>[2x]MLYIDEFKEAIDKGYILGDTVAIVRKNGKIFDYVLPHEKVRDDEVVTVERVEEVMVELDKLEHHHHHH;> GSHMLKDFGKKIKSLRLEKGLTKEAVCLDESQLSTRQLTRIESGQSTPTLNKAVYIAGRLGVTLGYLTD

Within S. pyogenes, Prx functions to inhibit the quorum-sensing receptor-signal pair ComRS, the master regulator of natural competence, or the ability to uptake endogenous DNA. ComR is a quorum-sensing receptor and a transcription factor that belongs to the Rgg subgroup of the RRNPP protein family, many of which regulate virulence in pathogenic Streptococcus species. ComR is a monomer that contains a DNA-binding domain (DBD) packed against a tetratricopeptide repeat (TPR) domain. Specifically, Prx binds directly to the apo-form of ComR preventing DNA binding in vitro and acts as a repressor of the S. pyogenes competence regulon in vivo.

Despite not being able to obtain an X-ray crystal structure of Prx in complex with full-length ComR, we were able to cocrystallize Prx with the DBD of ComR. DBD:Prx cocrystals were obtained with both purified minimal DBD bound to Prx and after in situ proteolysis with full-length ComR complexed with Prx. The crystals grew in similar conditions and both diffracted to 1.65 Å and 1.60 Å, respectively. The obtained complexes are nearly identical except for differences in space group (P212121 and P41212) and their cloning and protease digestion artifacts. Analysis of the DBD:Prx complex interface reveals that Prx directly interacts with the DNA-binding surface of ComR. The interaction is highly electrostatic in nature, with Prx using a large negative surface consisting of conserved acidic residues to complement the conserved positive DNA-interaction face of the ComR DBD. Specifically, Prx utilizes D32 to make hydrogen bonds with both the essential arginine residues R33 and R37 in ComR that are responsible for DNA recognition. Furthermore, residue D32 is the focal point for a stabilized hydrogen bonding network that positions Prx E44 to make a salt-bridge with ComR R33, Prx D38 to salt-bridge with ComR R37 and for the arginine side chains to be further stabilized by hydrogen bond interactions with the Prx mainchain. This binding network is extended across the full face of the DBD:Prx interaction by Prx E6 making a hydrogen bond with the invariable ComR residue K49 and Prx E9 providing a mainchain hydrogen bond with ComR T44. If the DBD:Prx complex is aligned to apo-ComR using the DBD, we observed that Prx is unable to interact with the DNA-binding residues of ComR due to a large steric clash as this surface is held tightly against the TPR domain.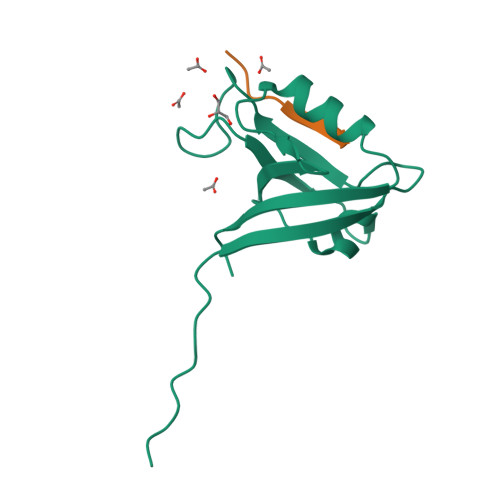>[2x]SAPSVKGVSFDQANNLLIEPARIEEEELTLTILRQTGGLGISIAGGKGSTPYKGDDEGIFISRVSEEGPAARAGVRVGDKLLEVNGVALQGAEHHEAVEALRGAGTAVQMRVWRERM;>[2x]KHFRETEV>GSHMDSTTIQQNKDTLSQIVVFPTGNYDKNEANAMVNRLANIDGKYLNALKQNNLKIKLLSGKLTDEKEYAYLKGVVPKGHEGTGKTWDDVPGLGGSTVALRIGFSNKGKGHDAINLELHATAHAIDHIVLNDISKSAQFKQIFAKEGRSLGNVNFLGVYPEEFFAESFAYYYLNQDTNSKLKSACPQTYSFLQNLAK[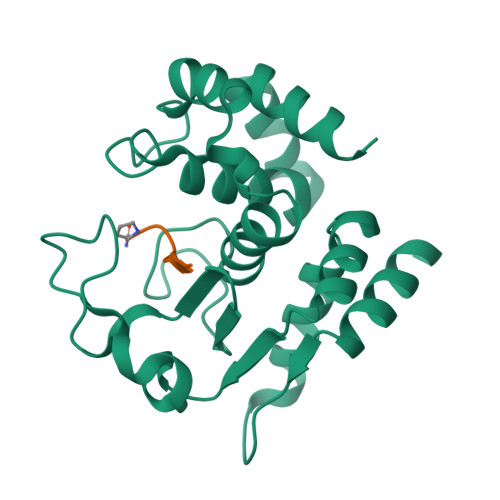2x];>XEVNPPVP[2x]>[4x]SNAMLLGAWDNAYIAAAMPLLLLVENIRSWPTRNAAEVRPPIVRELQYFQQHLQKKNYPQEDINHLSYLLCTYIDGIFNGLQTPDSYNQSLLVEFHRD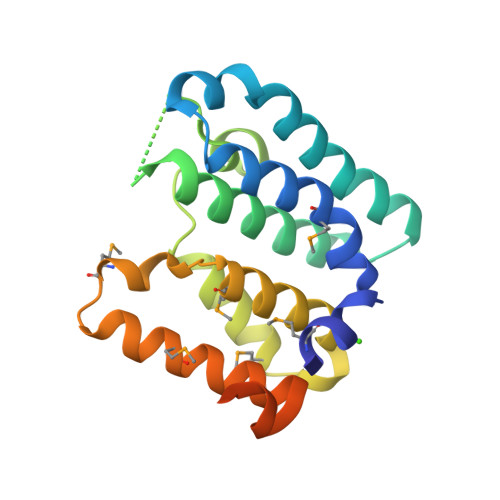AWGGEDCFEHLRVYMNSPKQYREVLEFYDLIMCLGFDGKYQMIEHGAVLLMDLRSRLHTQLYGQDATQSLAIAQAVKGSPRRQYIKALKIFT CASUARINE | C8 H15 N O5 | 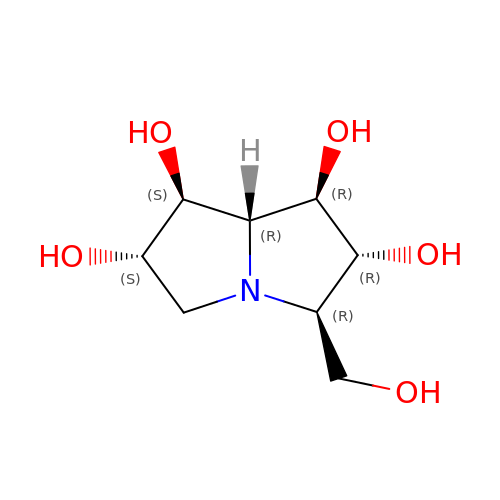AXTGOJVKRHFYBT-XAZAIFFQSA-N> MNRIKVAILFGGCSEEHDVSVKSAIEIAANINKEKYEPLYIGITKSGVWKMCEKPCAEWENENCYSAVLSPDKKMHGLLVKKNHEYEINHVDVAFSALHGKSGEDGSI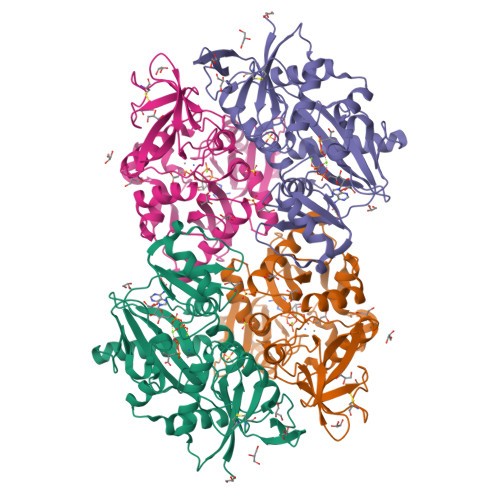QGLFELSGIPFVGCDIQSSAICMDKSLTYIVAKNAGIATPAFWVINKDDRPVAATFTYPVFVKPARSGSSFGVKKVNSADELDYAIESARQYDSKILIEQAVSGCEVGCAVLGNSAALVVGEVDQIRLQYGIFRIHQEVEPEKGSENAVITVPADLSAEERGRIQETVKKIYKTLGCRGLARVDMFLQDNGRIVLNEVNTLPGFTSYSRYPRMMAAAGISLPELIDRLIVLALKG;> MNRIKVAILFGGCSEEHDVSVKSAIEIAANINKEKYEPLYIGITKSGVWKMCEKPCAEWENENCYSAVLSPDKKMHGLLVKKNHEYEINHVDVAFSALHGKSGEDGSIQGLFELSGIPFVGCDIQSSAICMDKSLTYIVAKNAGIATPAFWVINKDDRPVAATFTYPVFVKPARSGSSFGVKKVNSADELDYAIESARQYDSKILIEQAVSGCEVGCAVLGNSAALVVGEVDQIRLQYGIFRIHQEVEPEKGSENAVITVPADLSAEERGRIQETVKKIYKTLGCRGLARVDMFLQDRGRIVLNEVNTLPGFTSYSRYPRMMAAAGISLPELIDRLIVLALKG>[2x]MAPRNEIEETLVTIWQDVLGIEKIGIKDNFYALGGDSIKAIQVAARLHSYQLKLETKDLLKYPTIDQLVHYIKDSKRRSEQGIVEGEIGLTPIQHWFFEQQFTNMHHWNQSYMLYRPNGFDKEILLRVFNKIVEHHDALRMIYKHHNGKIVQINRGLEGTLFDFYTFDLTANDNEQQVICEESARLQNSINLEVGPLVKIALFHTQNGDHLFMAIHHLVVDGISW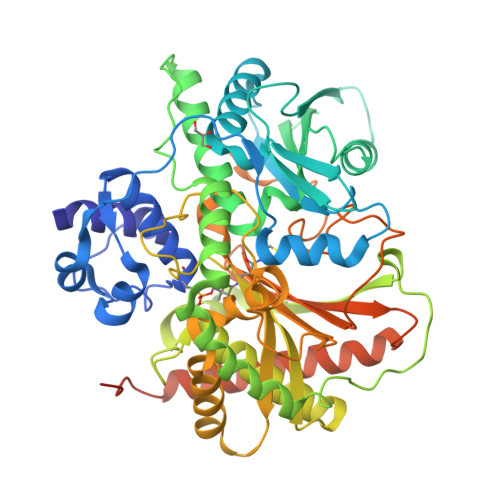RILFEDLATAYEQAMHQQTIALPEKTDSFKDWSIELEKYANSELFLEEAEYWHHLNYYTDNVQIKKDYVTMNNKQKNIRYVGMELTIEETEKLLKNVNKAYRTEINDILLTALGFALKEWADIDKIVINLEGHGREEILEQMNIARTVGWFTSQYPVVLDMQKSDDLSYQIKLMKENLRRIPNKGIGYEIFKYLTTEYLRPVLPFTLKPEINFNYLGQFDTDVKTELFTRSPYSMGNSLGPDGKNNLGPEGESYFVLNINGFIEEGKLHITFSYNEQQYKEDTIQQLSRSYKQHLLAIIEHCVQKEDTELTPSDFSFKELELEEMDDIFDLLADSLTDDDDKHHHHHH>[6x]MRSIITQICNGVLHGQSYQSGSNDLDKGNSEIFASSLFVHLNEQGKEIIKHKDSDDKIVIGYTKDGMAFQIVVDGFYGCERQAVFSFIDNYVLPLIDNFSLDLTRYPDSKKVTESLIHTIYSLRSKHAPLAEFTMSLCVTYQKDEQLFCAGFGIGDTGIAIKRNEGTIEQLVCHTEVDGFKDAFDNYSSANIDLVIERNSVFNTKVMPGDELVGYTYVPPMLEMTEKEFEVETVDGKKINKRIVRHLNLDPGNFDDKDPLFSQLLQVVKSKQKQLVEQAKETGQIQRFGDDFTVGRLVIPDQLLINQLRIHALSIGVSDGLLSYIKNENENKGFLGIYGFFTGADKNIEKATLYKNLIAKYQNNHFISLIILSALVSDSKTPLMTQYLVGYLDFPSKALLANKITELLLKELENPDMREILGSRLATDVIEELETKIIRYIHNPAGSDIHSTLNLWTADKIKAATNSSLTI

While SidM catalyzes the attachment of adenosine monophosphate (AMP) to Rab1, SidD catalyzes AMP removal from Rab1, a process known as deAMPylation. Inactivation and removal of Rab1 is initiated upon translocation of the effector SidD which deAMPylates Rab1, thereby priming it for inactivation by the L. pneumophila GAP LepB and causing its gradual removal from the LCV 4–6 hours after bacterial uptake. SidD is a protein of 507 amino acids with no significant sequence homology to other entries in the database. Taken together, our data revealed that the CTD mediates localization of SidD to membranes using a dual-binding mode that combines a general membrane-binding determinant in form of the loopCTD with a specificity determinant represented by a helix-turn-helix unit at the C-terminus.

Crystals that diffracted to 3.6 Å were obtained with a slightly truncated variant comprised of residues 37–507 (SidD37-507). Residues 85–88, 269–276, 365–382 and 495–507 were not well-defined in the electron density map and could not be modeled. The six SidD37-507 molecules present in the asymmetric unit displayed identical structures with an L-like shape formed by two domains in nearly perpendicular orientation. The N-terminal deAMPylase domain possesses a protein phosphatase fold, while the CTD is formed by a bundle of anti-parallel alpha-helices with no apparent similarity to known structures. The two domains are connected via a flexible linker and are positioned almost perpendicular to each other in the crystal lattice. The ab initio molecular envelope calculated from the SAXS data revealed a similar L-shaped structure but with a maximum diameter Dmax of 115 Å, which differed from the calculated value of 89.2 Å for the crystal structure. Indeed, the SidD37-507 crystallographic structure exhibited a low fit with the observed solution scattering curve (χ2 = 2.48) supporting the hypothesis of interdomain flexibility. Our SAXS analyses subsequently revealed a relative mobility between the two domains, with 76% of the particles existing as L-shaped molecules in solution while the other 24% of the particles assumed a more extended morphology. Upon closer examination of the CTD sequence, we noticed a stretch of hydrophobic residues between helices α7 and α8 (370-FLGIYGFFT-378; loopCTD) that was unstructured in the crystal structure of SidD37-507, indicative of intrinsic flexibility, and that could constitute a potential membrane anchor for SidD. Having a high degree of flexibility between the catalytic domain and the localization domain could increase the sampling radius of membrane bound SidD from a two-dimensional plane to a three-dimensional space.Here, we report that a nucleoid occlusion protein Noc is a CTPase enzyme whose membrane-binding activity is directly regulated by a CTP switch. In Bacillus subtilis, Noc nucleates on 16 bp NBS sites before associating with neighboring non-specific DNA to form large membrane-associated nucleoprotein complexes to physically occlude assembly of the cell division machinery. Unusually, Noc is also a peripheral membrane protein that directly associates with the cell membrane via a predicted N-terminal amphipathic helix (Adams et al., 2015). We provide evidence that (1) CTP is required for Noc to form the NBS-dependent nucleoprotein complex, and (2) CTP binding switches Noc from a membrane-inactive auto-repressed state to a membrane-active state.

However, in the presence of CTPɣS, we were able to grow and collect 2.95 Å diffraction data for a crystal of a further truncated G. thermoleovorans NocNΔ26ΔCTD variant, which lacks both the N-terminal membrane-targeting helix and the C-terminal domain. After solving its structure, it was apparent that NocNΔ26ΔCTD had adopted an alternative conformation to that of NocΔCTD (Figure 6A versus Figures 6B and 6C). However, there was no clear electron density for a bound nucleotide in our structure; instead a sulfate anion from the crystallization solution occupies a position equivalent to that of the β-phosphate of the nucleotide in the B. subtilis ParBΔCTD-CDP structure (Soh et al., 2019). We further observed that helix α5 in the NocΔN26ΔCTD structure swings outward by 104° and no longer forms a bundle with helix α6 from the same subunit (Figure 6A versus Figure 6B) and that this movement might drive the self-dimerization at the NTD of Noc (i.e., the NTD engagement). By superimposing the NTDs of NocΔCTD and NocNΔ26ΔCTD (RMSD = 1.49 Å), we detected severe clashes between α1, α2, and the opposite subunit of NocNΔ26ΔCTD. Therefore, it is clear that the autoinhibitory state of α1 and α2 (as observed in NocΔCTD) is not compatible with the alternative conformation in the NocNΔ26ΔCTD structure. The lack of a bound nucleotide in the NocNΔ26ΔCTD structure prevents us from drawing a conclusion on the role of CTP and the possible conformational liberation of the amphipathic helix α1. However, several lines of evidence suggest that CTP might favor the NTD-engagement conformation as observed in our NocNΔ26ΔCTD structure: (1) CTP/CTPɣS promoted the crosslinking between symmetrical E29C residues, a readout for NTD engagement; (2) the conformation of NocNΔ26ΔCTD is highly similar to that of a nucleotide-bound B. subtilis ParB (Soh et al., 2019); and (3) CTP/CTPɣS enables Noc (WT) to co-sediment with liposomes.

> MEEVRHIPVKSIIPNRFQPRTMFDEEKIDELALTIRTHGIIQPIVVRECGNGRFEIIAGERRWRAVQKLGWTEIPAIIKNLNDKETASVALIENLQREELTPIEEAMAYAKLIELHDLTQEALAQRLGKGQSTIANKLRLLKLPQEVQEALLQRAITERHARALIALKDKEKQLKLLQEIIDKQLNVKQTEDRVLKLLEAGERKPKPKRKAFSRDKLAAALEHHHHHH5-[7-(4-chlorophenyl)-1-methyl-6,7-dihydro-5H-[1,2,3]triazolo[1,5-d][1,4]benzodiazepin-9-yl]pyridin-2-amine | C22 H19 Cl N6 | 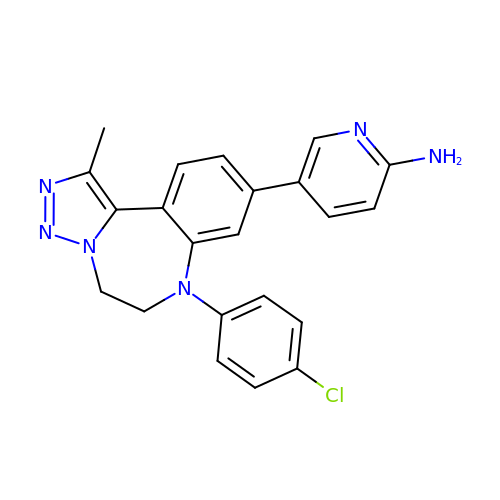PUTQASIWNBKTDJ-UHFFFAOYSA-N> MKTDFIMVPTAMPDEKMINYQLAIDGGEPVIPKANRKTIFPNIAKEDLFQMMISVQKPEEMVVSEFAEKYRQRVGAPYAIPTASGTSS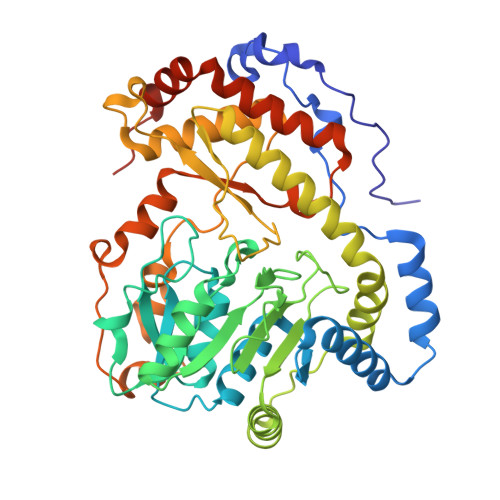LHLALVGAGVKAGDEVIVPAFTFIATAQAIVAAKAIPVFADIDPQTYCLDPRQLDKKVTARTKAVMPVHVHGLPADIDALASFCRQHQLALIEDASHAHSATLHGRYCGTFGDAAGQSLMADKNFPLGGEAGIAFFKERESYDRALAFLEESGLDYRMSWVAAAFGISQLDRLDYYDEIRQRNAQRLIDELATTRLFTGPMIPAAAKHSFNMFRIKINTALPEFKDIPEYKLKLALQQILNEEGVFAREWQNTLLPFHLPFQNKKGFGKGYPFFLGDSQEYKHEHFPNALQMLRSTLVLCRELRSPVEYEKLHSYIITFKKVDKNIQRVAEIASQIDDVPPYEKDARLGHHHHHH> MAAIPPDSWQPPNVYLETSMGIIVLELYWKHAPKTCKNFAELARRGYYNGTKFHRIIKDFMIQGGDPTGTGRGGASIYGKQFEDELHPDLKFTGAGILAMANA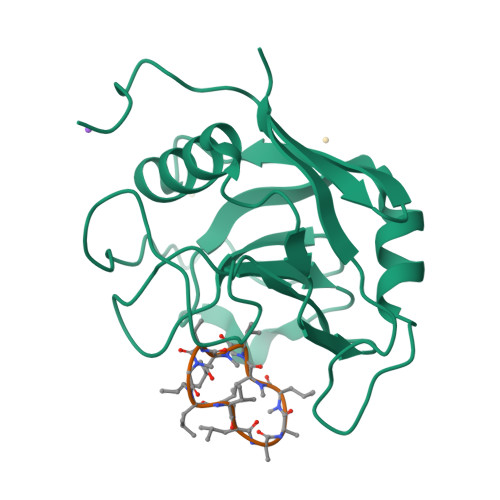GPDTNGSQFFVTLAPTQWLDGKHTIFGRVCQGIGMVNRVGMVETNSQDRPVDDVKIIKAYPSG;> ALLVTAGLVLA>[2x]MRLNPGQQQAVEFVTGPCLVLAGAGSGKTRVITNKIAHLIRGCGYQARHIAAVTFTNKAAREMKERVGQTLGRKEARGLMISTFHTLGLDIIKREYAALGMKANFSLFDDTDQLALLKELTEGLIEDDKVLLQQLISTISNWKNDLKTPSQAAASAIGERDRIFAHCYGLYDAHLKACNVLDFDDLILLPTLLLQANEEVRKRWQNKIRYLLVDEYQDTNTSQYELVKLLVGSRARFTVVGDDDQSIYSWRGARPQNLVLLSQDFPALKVIKLEQNYRSSGRILKAANILIANNPHVFEKRLFSELGYGAELK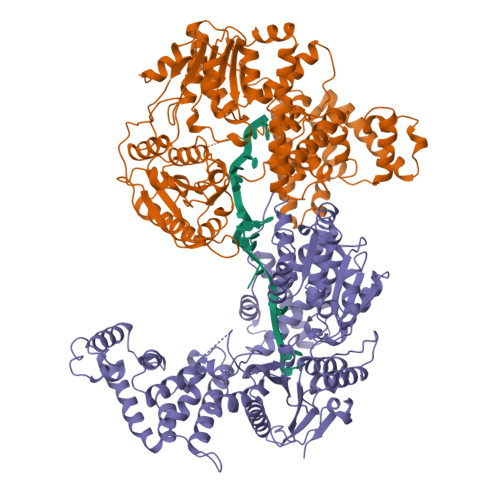VLSANNEEHEAERVTGELIAHHFVNKTQYKDYAILYRGNHQSRVFEKFLMQNRIPYKISGGTSFFSRPEIKDLLAYLRVLTNPDDDSAFLRIVNTPKREIGPATLKKLGEWAMTRNKSMFTASFDMGLSQTLSGRGYEALTRFTHWLAEIQRLAEREPIAAVRDLIHGMDYESWLYETSPSPKAAEMRMKNVNQLFSWMTEMLEGSELDEPMTLTQVVTRFTLRDMMERGESEEELDQVQLMTLHASKGLEFPYVYMVGMEEGFLPHQSSIDEDNIDEERRLAYVGITRAQKELTFTLCKERRQYGELVRPEPSRFLLELPQDDLIWEQERKVVSAEERMQKGQSHLANLKAMMAAKRGK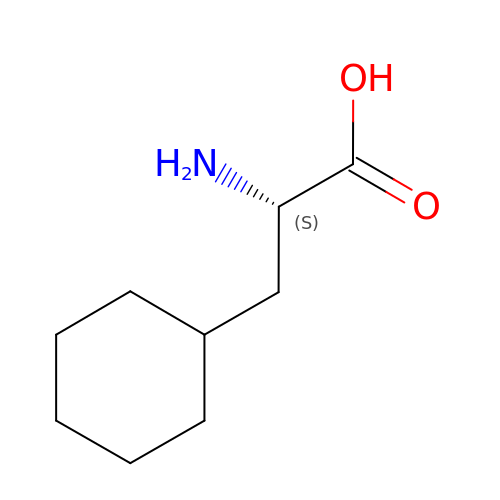2-AMINO-3-CYCLOHEXYL-PROPIONIC ACID | C9 H17 N O2 | ORQXBVXKBGUSBA-QMMMGPOBSA-N> SNARDPRPLRDKNFQSAIQEEIYDYLKKNKFDIETNHPISIKFLKQPTQKGFIIIFKWLYLRLDPGY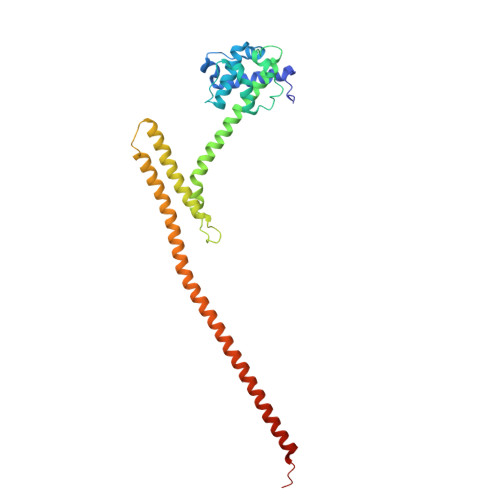GFTKSIENEIYQILKNLRYPFLESINKSQISAVGGSNWHKFLGMLHWMVRTNIKLDMCLNKVDRSLINQNTQEITILSQPLKTLDEQDQRQERYELMVEKLLIDYFTESYKSFLKLEDNYEPSMQELKLGFEKFVHIINTDVTSTELKLEELKVDLNRKRYKLHQQVIHVIDITSKFKINIQSSLENSENELGNVIEELRNLEFETEHNV>[2x]MVHYYRLSLKSRQKAPKIVNS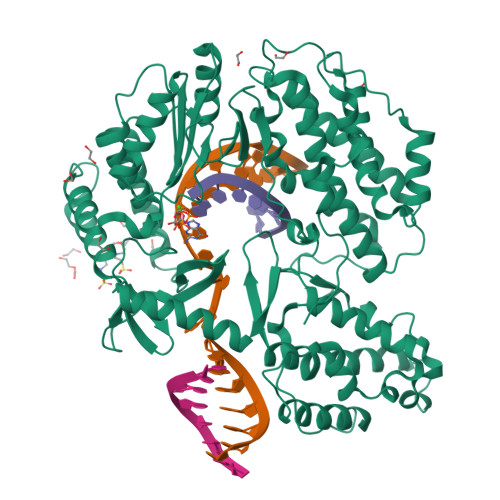KYNSILNIALKNFRLCKKHKTKKPVQILALLQEIIPKSYFGTTTNLKRFYKVVEKILTQSSFECIHLSVLHKCYDYDAIPWLQNVEPNLRPKLLLKHNLFLLDNIVKPIIAFYYKPIKTLNGHEIKFIRKEEYISFESKVFHKLKKMKYLVEVQDEVKPRGVLNIIPKQDNFRAIVSIFPDSARKPFFKLLTSKIYKVLEEKYKTSGSLYTCWSEFTQKTQGQIYGIKVDIRDAYGNVKIPVLCKLIQSIPTHLLDSEKKNFIVDHISNQFVAFRRKIYKWNHGLLQGDPLSGCLCELYMAFMDRLYFSNLDKDAFIHRTVDDYFFCSPHPHKVYDFELLIKGVYQVNPTKTRTNLPTHRHPQDEIPYCGKIFNLTTRQVRTLYKLPPNYEIRHKFKLWNFNNQISDDNPARFLQKAMDFPFICNSFTKFEFNTVFNDQRTVFANFYDAMICVAYKFDAAMMALRTSFLVNDFGFIWLVLSSTVRAYASRAFKKIVTYKGGKYRKVTFQCLKSIAWRAFLAVLKRRTEIYKGLIDRIKSREKLTMKFHDGEVDASYFCKLPEKFRFVKINRKASI>[4x]MNELVDTTEMYLRTIYDLEEEGVTPLRARIAERLDQSGPTVSQTVSRMERDGLLRVAGDR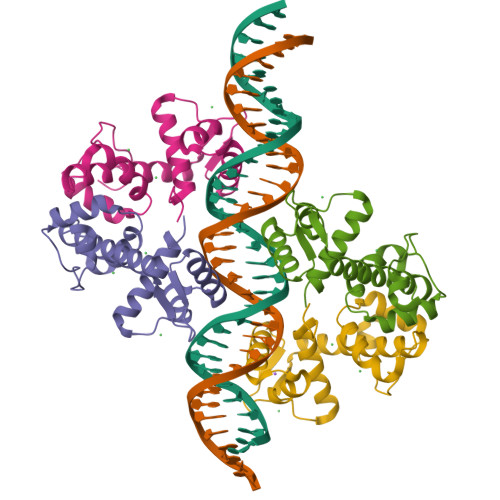HLELTEKGRALAIAVMRKHRLAERLLVDVIGLPWEEVHAEACRWEHVMSEDVERRLVKVLNNPTTSPFGNPIPGLVELGVASENLYFQGGGHHHHHH> ADQENSPLHTVGFDARFPQQNQTKHCWQSY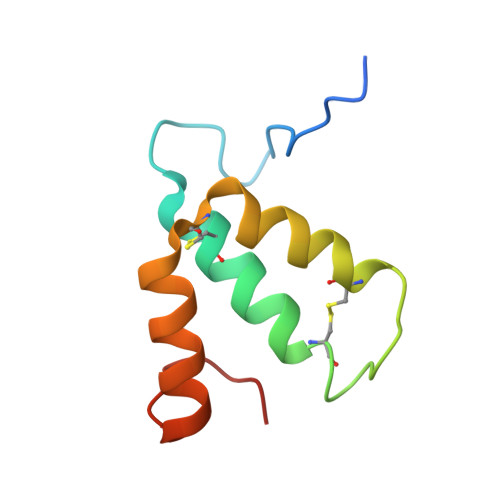VDYHKCVNMKGEDFAPCKVFWKTYNALCPLDWIEKWDDQREKGIFAGDINSD1-(4-IODOBENZOYL)-5-METHOXY-2-METHYL 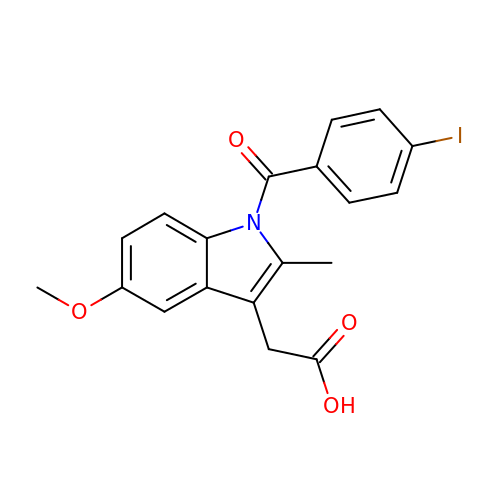INDOLE-3-ACETIC ACID | C19 H16 I N O4 | CXBFZYKAVCAPSV-UHFFFAOYSA-N>[24x]VEEVIEMQGLSLDPTSHRVMAGEEPLEMGPTEFKLLHFFMTHPERVYSREQLLNHVWGTNVYVEDRTVDVHIRRLRKALEPGGHDRMVQTVRGTGYRFSTRF;>MDSA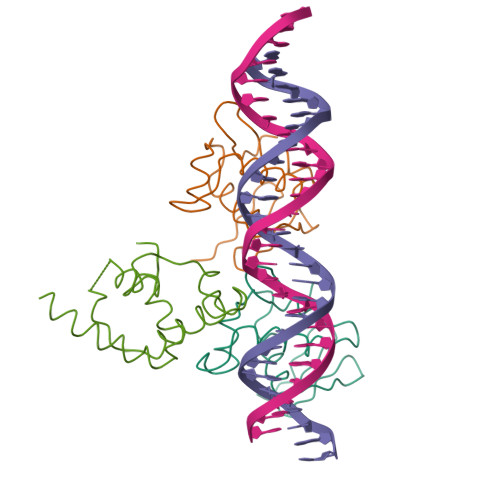TTESLRAATHDVLAGLTAREAKVLRMRFGIDMNTDYTLEEVGKQFDVTRERIRQIEAKALRKLRHPSRSEVLRSGSSGSGTPEEKLLRAIFGEKA[2x]> TEDEIRKLKKLLEEAEKKLYKLEDKTRRSEEISKTDDDPKAQSLQLIAESLMLIAESLLIIAISL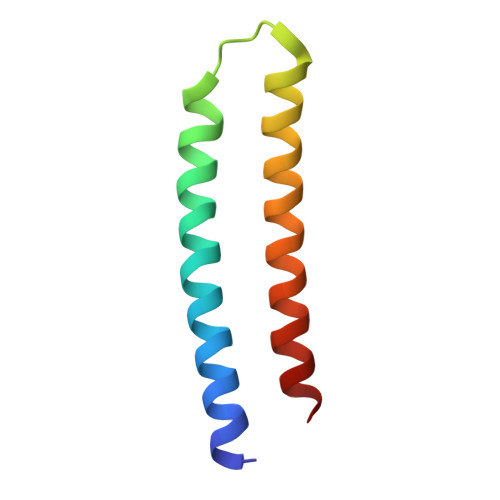LLSS Herein we have identified eight Sus-like systems in B. thetaiotaomicron that share the feature of a homologous SusE-like factor encoded immediately downstream from the transporter/lipoprotein duo susC/D. Two SusE-like proteins from these systems, BT2857 and BT3158, were characterized by X-ray crystallography and BT2857 was further analyzed by small-angle X-ray scattering. The SusE-like proteins were found to be composed of a conserved three domain architecture: a partially disordered N-terminal domain that is predicted to be proximal to the membrane and structurally homologous to an FN3-like bundle, a middle β-sandwich domain, and a C-terminal domain homologous to family 32 carbohydrate-binding modules, that bind to galactose. However, functional analyses with BT2857 and BT3158 revealed that the SusE-like proteins exhibited galactosidase activity with para-nitrophenyl-β-D-galactopyranoside and α-(1,4)-lactose substrates, that has not been demonstrated for SusE proteins. Using a series of domain truncations of BT2857, the predominant β-D-galactosidase activity is suggested to be localized to the C-terminal DUF5126 domain that would be most distal from the outer membrane.

BT3158 crystallized in a C21 space group, with one molecule in the asymmetric unit. Diffraction data for BT3158 were processed to a maximum resolution of 1.50 Å. Despite performing diffraction analyses on multiple crystals and no detectable protein degradation observed via SDS-PAGE, discontinuous electron density was characteristic across the majority of the N-terminal DUF4959 domain. Iterative rebuilding and refinement of this region suggested that it is composed mainly of β-strands, consistent with sequence-based homology modeling as an FN3-like bundle domain. This deficiency in electron density across the N-terminal region and sufficient size of the asymmetric unit to accommodate the domains was similar to results seen in the prototypical SusE and Ea domain of BT3700; thereby suggesting this region is consistently disordered and likely forms a discrete domain that would reside close to the membrane and have flexibility independent of the rest of the protein. Beyond the membrane-proximal DUF4959 partially disordered domain, BT3158 presented a distinct two-domain structure, with backbone residues confidently modeled with the exception of an extended loop (166–173). Structures of the DUF5000 or Ec domains (BT2857C and BT3158E223–P440) were compared via the MatchMaker in Chimera using the Smith-Waterman algorithm, yielding a RMSD of 1.225 Å across C-alpha atoms, and a quality score of 0.768. In BT3158 an ethylene glycol and H265 are also structurally conserved. However, this is where the similarities at this region stop in that in BT3158 A304 is in a structurally equivalent position to D304, and none of the other residues between these proteins are conserved in this region suggesting sequence and structural divergence that could also reflect functional variance.

> CEDVETHKPYGDGSGHAPGTVQVTSYEQIPGGVTLKFIAPTDEDLLYIKIKYTLDNGKEMEARASLYTDETTIEGFGNTNPKKLVISAVNKMEKEGEAIITEIVPGKPAYLTAIEEIEVNPTFGGIYIHTTNGGRNYLIFDVSTKDSKGNWNIEHTEYTSVKNIGFTLRGFSAEPHDFKVRVRDLYDNQSEEYLTTLTPLYEEKLDLTKFKTFYLANDIKMDNAGHTLESLFNGDHGLNSWNYAHGYDFNPSEFPVWFTFDMGQTAQLSRFTSWQRSMGGSYYYRAGAIKEWEVWGRSDLPSSDGSWDGWTKLADCESIKPSGWPTGSNSEEDITYASKGEEFEFLADIPPVRYIRFKILSTHDGAGLVVMQQLWFYGTPIQ> MDWLLATPQLYSAFSSLGCLEGDTYVVNPNALAILEEINYKLTYEDQTLRTFRRAIGFGQNVRSDLIPLLENAKDDAVLESVIRILVNLTVPVECLFSVDVMYRTDVGRHTIFELNKLLYTSKEAFTEARSTKSVVEYMKHILESDPKLSPHKCDQINNCLLLLRNILHIPETHAHCVMPMMQSMPHGISMQNTILWNLFIQSIDKLLLYLMTCPQRAFWGVTMVQLIALIYKDQHVSTLQKLLSLWFEASLSESSEDNESNTSPPKQGSGDSSPMLTSDPTSDSSDNGSNGRGMGGGMREGTAATLQEVSRKGQEYQNAMARVPADKPDGSEEASDMTGNDSEQPGSPEQSQPAGESMDDGDYEDQRHRQLNEHGEEDEDEDEVEEEEYLQLGPASEPLNLTQQPADKVNNTTNPTSSAPQGCLGNEPFKPPPPLPVRASTSAHAQMQKFNESSYASHVSAVKLGQKSPHAGQLQLTKGKCCPQKRECPSSQSELSDCGYGTQVENQESISTSSNDDDGPQGKPQHQKPPCNTKPRNKPRTIMSPMDKKELRRKKLVKRSKSSLINMKGLVQHTPTDDDISNLLKEFTVDFLLKGYSYLVEELHMQLLSNAKVPIDTSHFFWLVTYFLKFAAQLELDMEHIDTILTYDVLSYLTYEGVSLCEQLELNARQEGSDLKPYLRRMHLVVTAIREFLQAIDTYNKVTHLNEDDKAHLRQLQLQISEMSDLRCLFVLLLRRFNPSIHSKQYLQDLVVTNHILLLILDSSAKLGGCQTIRLSEHITQFATLEVMHYYGILLEDFNNNGEFVNDCIFTMMHHIGGDLGQIGVLFQPIILKTYSRIWEADYELCDDWSDLIEYVIHKFMNTPPKSPLTIPTTSLTEMTKEHNQEHTVCSWSQEEMDTLYWYYVQSKKNNDIVGKIVKLFSNNGNKLKTRISIIQQLLQQDIITLLEYDDLMKFEDAEYQRTLLTTPTSATTESGIEIKECAYGKPSDDVQILLDLIIKENKAQHLLWLQRILIECCFVKLTLRSGLKVPEGDHIMEPVAYHCICKQKSIPVVQWNNEQSTTMLYQPFVLLLHKLGIQLPADAGSIFARIPDYWTPETMYGLAKKLGPLDKLNLKFDASELEDATASSPSRYHHTGPRNSLSSVSSLDVDLGDTEELALIPEVDAAVEKAHAMASTPSPSEIFAVPKTKHCNSIIRYTPDPTPPVPNWLQLVMRSKCNHRTGPSGDPSDCIGSSSTTVDDEGFGKSISAATSQAASTSMSTVNPTTTLSLNMLNTFMGSHNENSSSSGCGGTVSSLSMVALMSTGAAGGGGNTSGLEMDVDASMKSSFERLEVNGSHFSRANNLDQEYSAMVASVYEKEKELNSDNVSLASDLTRMYVSDEDDRLERTEIRVPHYHLEGGSGMDKDCEMKRTTLDSPLGKLELSGCEQGLHRIIFLGKGTSAADAVEVPAPAAVLGGPEPLMQATAWLNAYFHQPEAIEEFPVPALHHPVFQQESFTRQVLWKLLKVVKFGEVISYSH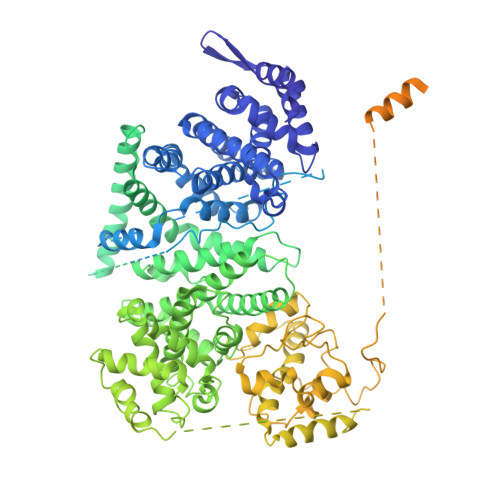LAALAGNPAATAAVKTALSGNPVPILIPCHRVVQGDLDVGGYEGGLAVKEWLLAHEGHRLGKPGLGGGGYPYDVPDYARTGGGSGSRLEEELRRRLTE>MELIQDTSRPPLEYVKGVPLIKYFAEALGPLQSFQARPDDLLINTYPKSGTTWVSQILDMIYQGGDLEKCNRAPIYVRVPFLEVNDPGEPSGLETLKDTPP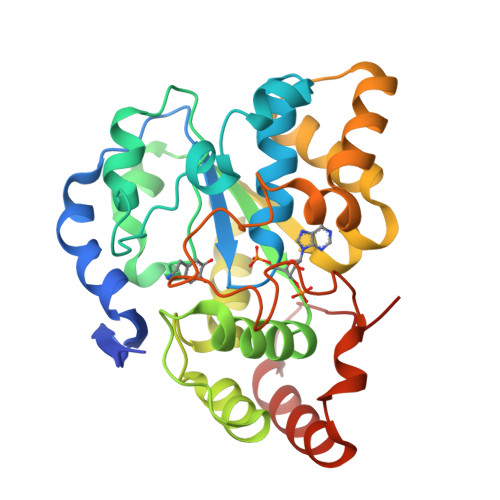PRLIKSHLPLALLPQTLLDQKVKVVYVARNPKDVAVSYYHFHRMEKAHPEPGTWDSFLEKFMAGEVSYGSWYQHVQEWWELSRTHPVLYLFYEDMKENPKREIQKILEFVGRSLPEETMDFMVQHTSFKEMKKNPMTNYTTVPQELMDHSISPFMRKGMAGDWKTTFTVAQNERFDADYAEKMAGCSLSFRSEL[2x]> MRILEEDLKNSTYRIRIESLDDLWYLRNILSEGDEVSAITFRRVEESADVQRSRERERIPITIRLKVEKIEFQDFDNRLRILGTVI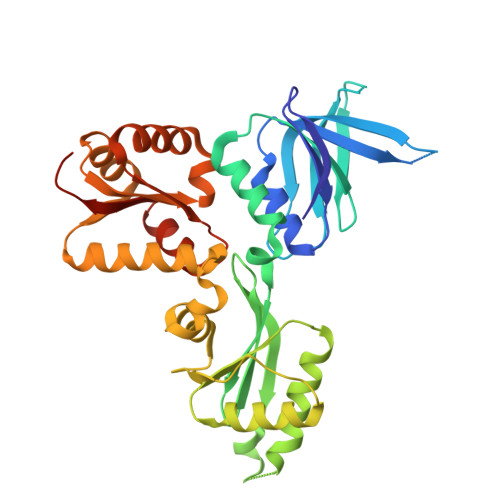EGPEDTKGKHQSITVTVDSEISITKEWDDQHIDLLKEATDEKYVTVYTAVAMDEDEAQIFLIHPYGIQQVGTVYSGRSGKYAEGNYSEASYFDQIVNALKNYSNSIIILGPGFARDRFARYCAQRGVNVIGSFPANRTDSGAVYEFITSADGAKLLSNERIARDKEIVDEFLVAVKKDMGVYGRDQTESALQMGALSDLIITDEMFRTEDGRRSLSIAQTVGTRIHIVSVSNDPGQIVKKFGGFAGILRYRVQLEHHHHHH> TQNFIIPKKEIHTVPDMGKWKRSQAYADYIGFILTLNEGVKGKKLTFEYRVSEAIEKLLALLNTLDR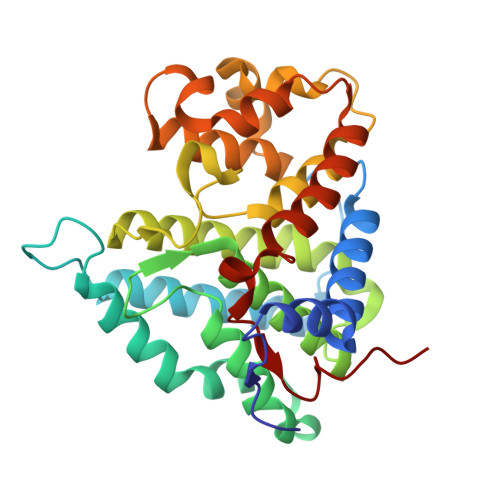WIDETPPVDQPSRFGNKAYRTWYAKLDEEAENLVATVVPTHLAAAVPEVAVYLKESVGNSTRIDYGTGHEAAFAAFLCCLCKIGVLRVDDQIAIVFKVFNRYLEVMRKLQKTYRMEPAGSQGVWGLDDFQFLPFIWGSSQLIDHPYLEPRHFVDEKAVNENHKDYMFLECILFITEMKTGPFAEHSNQLWNISAVPSWSKVNQGLIRMYKAECLEKFPVIQHFKFGSLLPIHPVTS>[2x]MHHHHHHSSGRENLYFQGKLPEPQFYAEPHTYEEPGRAGRSFTREIEASRIHIEKIIGSGDSGEVCYGRLRVPG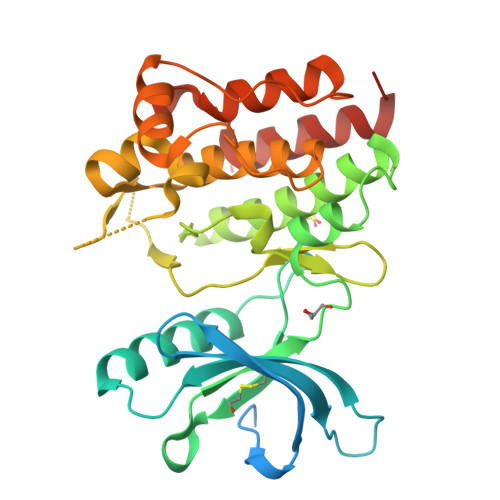QRDVPVAIKALKAGYTERQRRDFLSEASIMGQFDHPNIIRLEGVVTRGRLAMIVTEYMENGSLDTFLRTHDGQFTIMQLVGMLRGVGAGMRYLSDLGYVHRDLAARNVLVDSNLVCKVSDFGLSRVLEDDPDAAYTTTGGKIPIRWTAPEAIAFRTFSSASDVWSFGVVMWEVLAYGERPYWNMTNRDVISSVEEGYRLPAPMGCPHALHQLMLDCWHKDRAQRPRFSQIVSVLDALIRSPESLRATATVS>[2x]MLYHLFVNNQVKLQNDFKPESVAAIRSSAFNSKGGTTVFNFLSAGENILLHISIRPGENVIVFNSRLKNGAWGPEE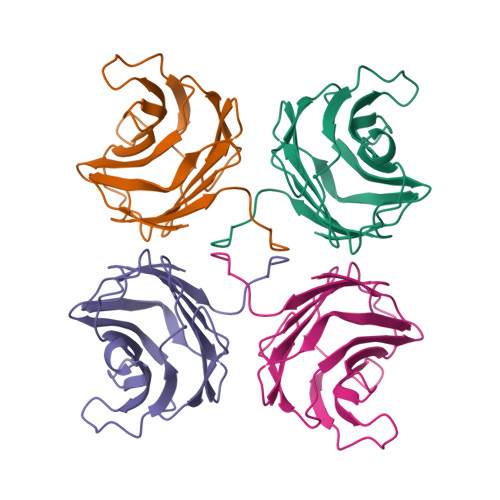RIPYAEKFRPPNPSITVIDHGDRFQIRFDYGTSIYYNKRIKENAAAIAYNAENSLFSSPVTVDVHGLLPPLPPA>[4x]MRGSHHHHHHENLYFQGSPRWILGDKFDTVFPHKGSLKVLWESRWKFACSKSVYPFHDGSIEDFEPIFNHLISKNINDAASDEYTQAFLPTASALEEKAAQALQAGKHEEASNLLCRAAVVYRISRFPYVDITKPNSIKRVAFERQKQAYLKATSLWTQPIREVTVPHTYRTGN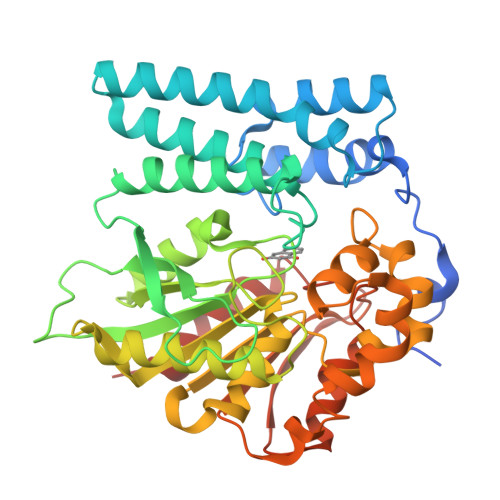DGAHIPIYIRTPAGADQSNPVPIVLIMTGLDGYRPDNSQRTHEILARGWAAVVAEIPGTADCPADPADPASPDRLWDSVLSYLDQRPELNTAKMVVWGLSAGGYYAIRAAHTHRDRLLGAIAHGPGCHYYLDPEWLAKVNDHEYPFEITAAWATKHGYKTVEEFVAGAQKKFSLVETGIVDQPSCRLLLLNGVDDGVVPIEDCLVLFEHGSPKEGRFYKGLPHMGYPNSLPVSYEWLEQVLASPSKTKN>MRVPEKYSTLPAEDRSVHIVNICAIEDLGYLPSEGTLLNSLSVDPDAECKYGLYFRDGKRKVDYILVYHHKRASGSRTLARRGLQNDMVLGTRSVRQDQPLPGKGSPVDAGSPEVPMDYHEDDKRFRREEYEGNLLEAGLELENDEDTKIHGVGFVKIHAPWHVLCREAEFLKLKMPTKKVYHISETRGLLKTINSVLQKITDPIQPKVAEHRPQTTKRLSYPFSREKQHLFDLTDRDSFFDSKTRSTIVYEILKRTTCTKAKYSMGITSLLANGVYSAAYPLHDGDYEGDNVEFNDRKLLYEEWASYGVFYKYQPIDLVRKYFGEKVGLYFAWLGAYTQMLIPASIVGVIVFLYGCATVDENIPSMEMCDQRYNITMCPLCDKTCSYWKMSSACATARASHLFDNPATVFFSVFMALWAATFMEHWKRKQMRLNYRWDLTGFEEEEDHPRAEYEARVLEKSLRKESRNKETDKVKLTWRDRFPAYFTNLVSIIFMIAVTFAIVLGVIIYRISTAAALAMNSSPSVRSNIRVTVTATAVIINLVVIILLDEVYGCIARWLTKIEVPKTEKS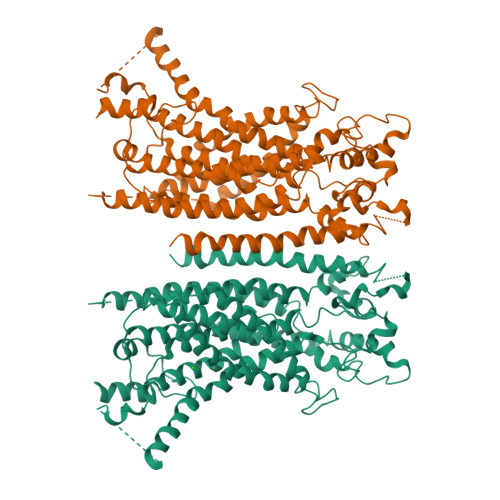FEERLTFKAFLLKFVNSYTPIFYVAFFKGRFVGRPGDYVYIFRSFRMEECAPGGCLMELCIQLSIIMLGKQLIQNNLFEIGIPKMKKFIRYLKLRRQSPSDREEYVKRKQRYEVDFNLEPFAGLTPEYMEMIIQFGFVTLFVASFPLAPLFALLNNIIEIRLDAKKFVTELRRPVAIRAKDIGIWYNILRGVGKLAVIINAFVISFTSDFIPRLVYLYMYSQNGTMHGFVNHTLSSFNVSDFQNGTAPNDPLDLGYEVQICRYKDYREPPWSEHKYDISKDFWAVLAARLAFVIVFQNLVMFMSDFVDWVIPDIPKDISQQIHKEKVLMVELSNSLEVLFQ[2x]> MSASAQQLAEELQIFGLDCEEALIEKLVELCVQYGQNEEGMVGELIAFCTSTHKVGLTSEILNSFEHEFLSKRLSKARHSTCKDSGHAGARDIVSIQELIEVEEEEEILLNSYTTPSKGSQKRAISTPETPLTKRSVSTRSPHQLLSPSSFSPSATPSQKYNSRSNRGEVVTSFGLAQGVSWSGRGGAGNISLKVLGCPEALTGSYKSMFQKLPDIREVLTCKIEELGSELKEHYKIEAFTPLLAPAQEPVTLLGQIGCDSNGKLNNKSVILEGDREHSSGAQIPVDLSELKEYSLFPGQVVIMEGINTTGRKLVATKLYEGVPLPFYQPTEEDADFEQSMVLVACGPYTTSDSITYDPLLDLIAVINHDRPDVCILFGPFLDAKHEQVENCLLTSPFEDIFKQCLRTIIEGTRSSGSHLVFVPSLRDVHHEPVYPQPPFSYSDLSREDKKQVQFVSEPCSLSINGVIFGLTSTDLLFHLGAEEISSSSGTSDRFSRILKHILTQRSYYPLYPPQEDMAIDYESFYVYAQLPVTPDVLIIPSE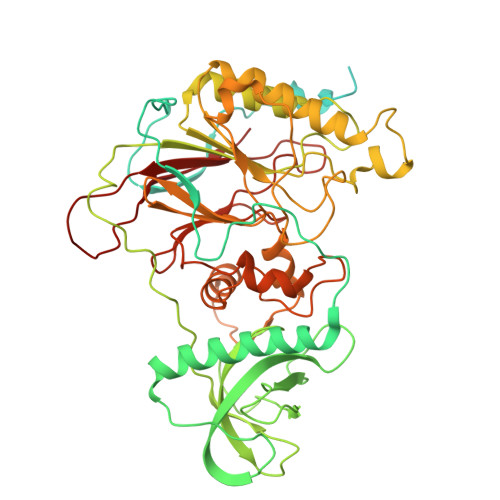LRYFVKDVLGCVCVNPGRLTKGQVGGTFARLYLRRPAADGAERQSPCIAVQVVRI>MATLFQVSMGSMRHRRNGNFESSRLLYSSMSRSIDVACSDADLANFIQENFKKRECVFFTKDTKSMGNLCKCGYPENQHIEGTQVNTTEKWNYKKXXXXXXXXXXXXXXXXXXXXXXKYIRLSCDTDSETLYDLMTQHWHLKTPNLVISVTGGAKNFALKPRMRKIFSRLIYIAQSKGAWIFTGGTHYGLMKYIGEVVRDNTISRSSEENVVAIGIAAWGMISNRETLIRTADSDGSYLAHYIMDDLKRDPLYCLDNNHTHLLLVDNGTHGHPTIEAKVRTQLEKYISERVIPESNYGGKIPIVCFAQGGGKETLKSINVAIKSKIPCVVVEGSGRIADVIASLVEAEGTLASSCVKESLLRFLPRTISRLSEEETESWIKWIKEVLESPHLLTVIKIEEAGDEIVSNAISFALYKAFSTNEHDRDNWNGQLKLLLEWNQLDLASDEIFTNDRNWESADLQDVMFTALVKDRPKFVRLFLENGLNLRKFLTTEVLRELYTNNFSSLVFKNLQIAKNSYNDALLTFVWKMVEDFRRGAKRDDKNSKDEMEIELSEECPITRHPLQALFIWSVLQNKKELSKVIWEQTRGCTLAALGASKLLKSMAKVKNDINAAGESEELANEYETRAVELFTECYSNDEDLAEQLLTYSCEAWGGSNCLELAVEARDQQFIAQPGVQNFLSKQWYGEISRDTKNWKIILCLFFFPLIGCGFISFRKKPVEKTKKLFLYYVSFFTSPFVVFSWNVIFYIAFLLLFAYVLLMDFQKEPTALEIILYVLVFILLCDEVRQWYMNGSKYFSDLWNVMDTLGIFYFIAGIVFRLHSDESSWYSGRVIFCLDYIVFTLRLIHIFTVSRNLGPKIIMLQRMMIDVFFFLFLFAVWMVAFGVARQGILRKNEHRWEWIFRSVIYEPYLAMFGQYPDDIDGTTYNFDHCTFSGNESKPLCVELDANNQPRFPEWITIPLVCIYMLSTNILLVNLLVAMFGYTVGSVQENNDQVWKFQRFFLVQEYCSRLTIPFPFVIFAYIFMVMRKCFKCCCKKESKEPSVCCSRN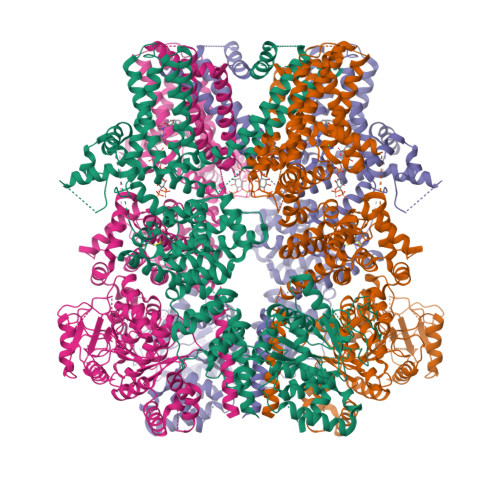EDNEILAWEAVMKENYLVKINTKASDSSEEXXXXXXXXXXXXXXXXXXXXXXXXKIKSNSLEVLFQGPDYKDDDDKAHHHHHHHHHH[4x]>[3x]MEDDDEEMQQKGCLERRYDTVCGFCRKHKTTLRHIIWGILLAGYLVMVISACVLNFHRALPLFVITVAAIFFVVWDHLMAKYEHRIDEMLSPGRRLLNSHWFWLKWVIWSSLVLAVIFWLAFDTAKLGQQQLVSFGGLIMYIVLLFLFSKYPTRVYWRPVLWGIGLQFLLGLLILRTDPGFIAFDWLGRQVQTFLEYTDAGASFVFGEKYKDHFFAFKVLPIVVFFSTVMSMLYYLGLMQWIIRKVGWIMLVTTGSSPIESVVASGNIFVGQTESPLLVRPYLPYITKSELHAIMTAGFSTIAGSVLGAYISFGVPSSHLLTASVMSAPASLAAAKLFWPETEKPKITLKNAMKMESGDSGNLLEAA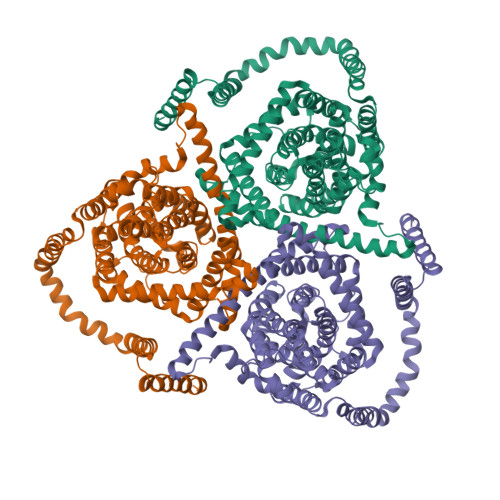TQGASSSISLVANIAVNLIAFLALLSFMNSALSWFGNMFDYPQLSFELICSYIFMPFSFMMGVEWQDSFMVARLIGYKTFFNEFVAYEHLSKWIHLRKEGGPKFVNGVQQYISIRSEIIATYALCGFANIGSLGIVIGGLTSMAPSRKRDIASGAVRALIAGTVACFMTACIAGILSSTPVDINCHHVLENAFNSTFPGNTTKVIACCQSLLSSTVAKGPGEVIPGGNHSLYSLKGCCTLLNPSTFNCNGISNTFLEWSHPQFEK>[12x]MTAPRSWAPTTRARGDTEALCSPEDGWVKVHPTPGTMLFREILHGQLGYTEGQGVYNVVRSSEATTRQLQAAIFHALLNATTYRDLEADWLGHVAARGLQPQRLVRRYRNAREADIAGVAERVFDTWRNTLRTTLLDFAHGLVACFAPGGPSGPSSFPKYIDWLTCLGLVPILRKRQEGGVTQGLRAFLKQHPLTRQLATVAEAAERAGPGFFELALAFDSTR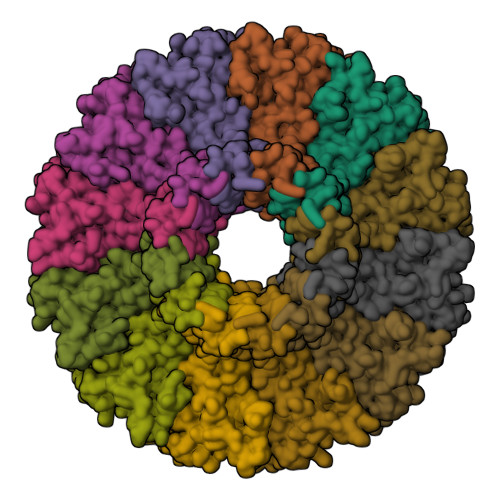VADYDRVYIYYNHRRGDWLVRDPISGQRGECLVLWPPLWTGDRLVFDSPVQRLFPEIVACHSLREHAHVCRLRNTASVKVLLGRKSDSERGVAGAARVVNKVLGEDDETKAGSAASRLVRLIINMKGMRHVGDINDTVRSYLDEAGGHLIDAPAVDGTLPGFGKGGNSRGSAGQDQGGRAPQLRQAFRTAVVNNINGVLEGYINNLFGTIERLRETNAGLATQLQERDRELRRATAGALERQQRAADLAAESVTGGCGSRPAGADLLRADYDIIDVSKSMDDDTYVANSFQHPYIPSYAQDLERLSRLWEHELVRCFKILCHRNNQGQETSISYSSGAIAAFVAPYFESVLRAPRVGAPITGSDVILGEEELWDAVFKKTRLQTYLTDIAALFVADVQHAALPPPPSPVGADFRPGASPRGRSRSRSPGRTAPGAPDQGGGIGHRDGRRDGRR> KPFKCSMCDYASVEVSKLKRHIRSHTGERPFQCSLCSYASRDTYKLKRHMRTHSGEKPYECYICHARFTQSGTMKMHILQKHTENVAKFHCPHCDTVIARKSDLGVHLRKQHSYIEQGKKCRYCDAVFHE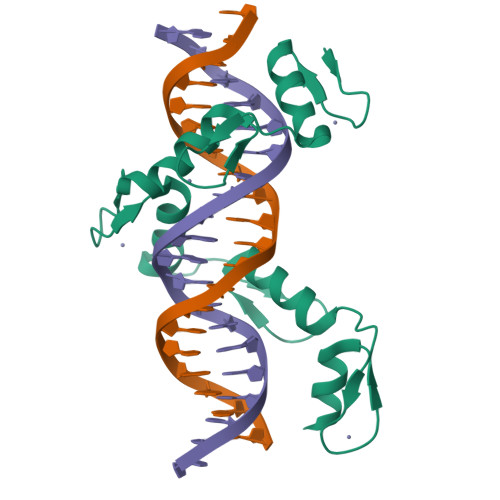RYALIQHQKSHK;> KPFKCSMCDYASVEVSKLKRHIRSHTGERPFQCSLCSYASRDTYKLKRHMRTHSGEKPYECYICHARFTQSGTMKMHILQKHTENVAKFHCPHCDTVIARKSDLGVHLRKQHSYIEQGKKCRYCDAVFHERYALIQHQKSH> MSHHHHHHHHHHDSNGIPTENLYFQGAGVAFGSFDDSFSLASLRAYLAEFISTLLFVFAGVGSAIAYA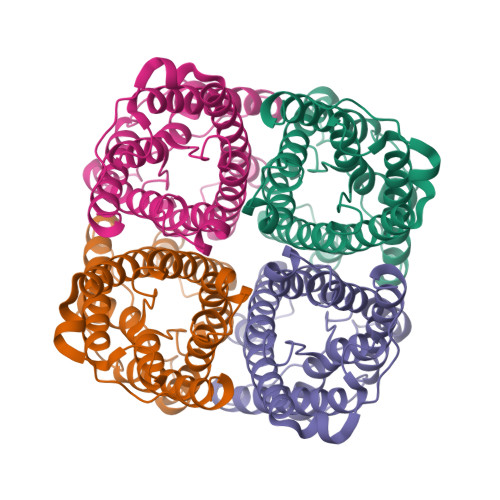KLTSDAALDTPGLVAIAVCHGFALFVAVAIGANISGGHVNPAVTFGLAVGGQITVITGVFYWIAQLLGSTAACFLLKYVTGGLAVPTHSVAAGLGSIEGVVMEIIITFALVYTVYATAADPKKGSLGTIAPLAIGLIVGANILAAGPFSGGSMNPARSFGPAVAAGDFSGHWVYWVGPLIGGGLAGLIYGNVFMGSSEHVPLASADF>[4x]SHGMAVTKVTVDGIEFPPTITPPGSSKSLTLLGAG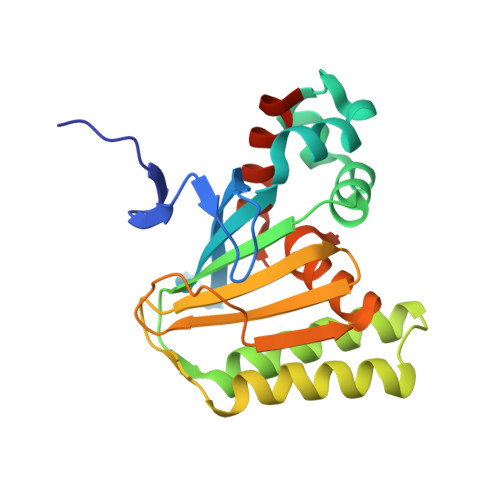VRGIEIETIQIKVTAIGVYAEPEVIASHLQKWKGKSASELVEDDGFFKDLVQAPVEKLAKITIIKGLKGSQYGGAVEENIRDRLAALDKYSEAEEEALEEFREFFKTKSLPKGSVIFFHWPSPSTLQISFSTDGSLPEEAEATVENANVAAALLDVFLGENSVSPSTKASVAEGISALLMKNKDEKEV> MLRITSACRGGYMMYHRKSMGTMKYSKWKGAHGGVSHFYGRTPMVEEVKRNEPITLIDRRIMHYVHRSRLRHFQLFRSYQQKSNATECKLREGEMLRRRWHRKLQKSFIAFMQFKTMKVLEDQAKLV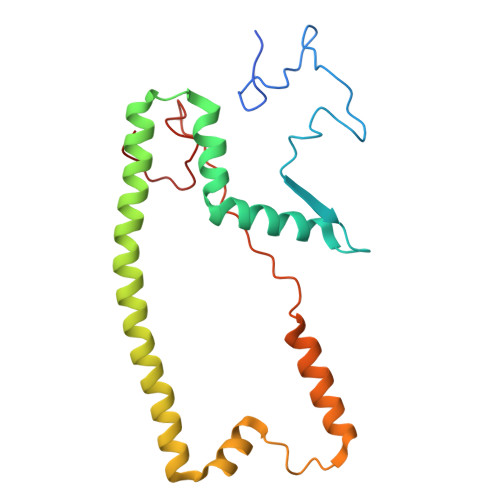NTYGQAAVNAALGDSWDAVSDKEKDRKYVTIRRQVKALPVVSVVPKHVATMKQIHNDRFNYRWRVN> GSSMKASSGDQGSPPCFLRFPRPVRVVSGAEAELKCVVLGEPPPVVVWEKGGQQLAASERLSFPADGAEHGLLLTAALPTDAGVYVCRARNAAGEA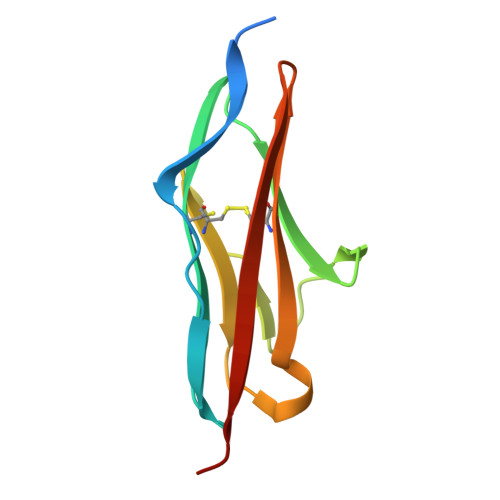YAAAAVTVLEPPA> GAMDSIQAEEWYFGKITRRESERLLLNAENPRGTFLVRESETVKGAYALSVSDFDNAKGLNVKHYLIRKLDSGGFYITSRTQFNSL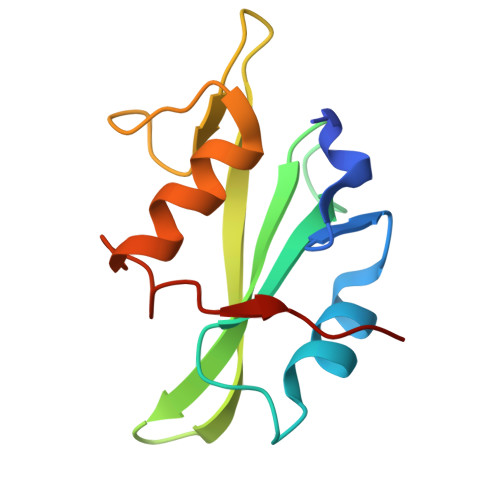QQLVAYYSKHADGLCHRLTTVCPTSK>MASVHGTTYELLRRQGIDTVFGNPGSNELPFLKDFPEDFRYILALQEACVVGIADGYAQASRKPAFINLHSAAGTGNAMGALSNAWNSHSPLIVTAGQQTRAMIGVEALLTNVDAANLPRPLVKWSYEPASAAEVPHAMSRAIHMASMAPQGPVYLSVPYDDWDKDADPQSHHLFDRHVSSSVRLNDQDLDILVKALNSASNPAIVLGPDVDAANANADCVMLAERLKAPVWVAPSAPRCPFPTRHPCFRGLMPAGIAAISQLLEGHDVVLVIGAPVFRYHQYDPGQYLKPGTRLISV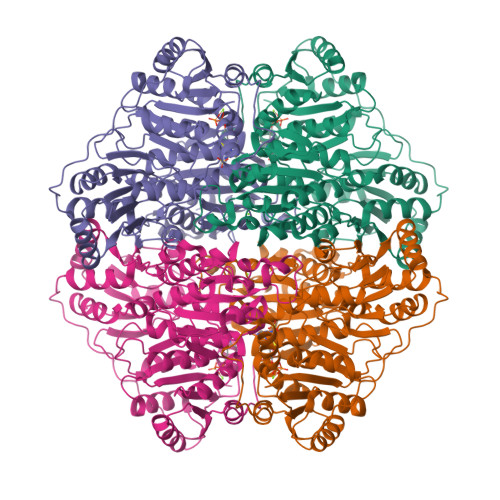TCDPLEAARAPMGDAIVADIGAMASALANLVEESSRQLPTAAPEPAKVDQDAGRLHPETVFDTLNDMAPENAIYLNESTSTTAQMWQRLNMRNPGSYYFCAAGGLGFALPAAIGVQLAEPERQVIAVIGDGSANYSISALWTAAQYNIPTIFVIMNNGTYGAARWFAGVLEAENVPGLDVPGIDFRALAKGYGVQALKADNLEQLKGSLQEALSAKGPVLIEVSTVSPVK[4x]>MSDHKPAGQFLDAAIDLLRRVRDEEADSIEAAGTLLADTVQNGGRLFAFGAGHSSLAAQDVVYRAGGLALMNLLTVPGVVGIDVMPATLGSALERVDGLASAVLDSSPLRAGDALVIISLSGRNALPVEMAMHARALGLRVIGVTSVAYASQTTSRHASGTFLKDHCDIVLDSKIAVGDAELTLDTVPAPFAPASTVVTAALMQAVTATAAATLADRGIEPPLLRSGNVDGGHEWNARV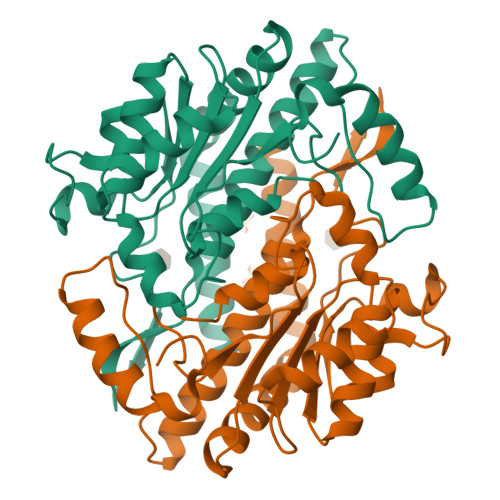LEQYGERIFYRR[2x]> SMAAAAVVQIPAGATFLETFKKSFVDVPIDAEKGNAISTAEFLEAAESLTTMFDVLGSIAFSPVKTDMLGNVEKIRKRML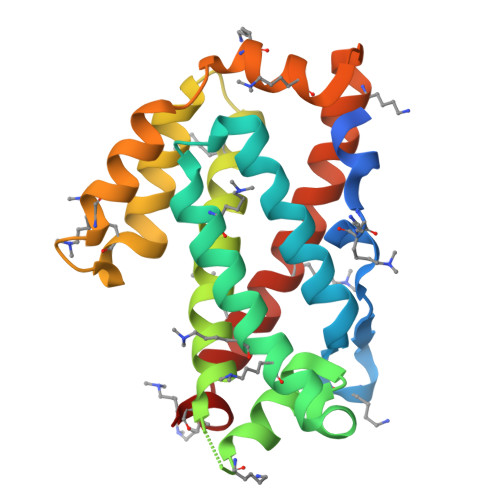AAPLESQNIQDLVRNELKTKSHTATEGLLWLVRGLEFTCIALSKNIGSTEELADSFRGSYRVTLKPHHSFLVKPIFSAAMSACPYRKDFYAKLGDDEQKVQEELREYLVALDKIVNILKRFLESKEAKW>GSHMAAELDSLLGQEKERFQVLPGRDKMLYVAAQNERDTLWARQVLARGDYDKNARVINENEENKRISIWLDTYYPQLAYYRIHFDEPRKPVFWLSRQRNTMSKKELEVLSQKLRALMPYADSVNITLMDDVTAAGQAEAGLKQQALPYSRRNHKGGVTFVIQGALDDVEILRARQFVDSYYRTWGGRYVQFAIELKDDWLKGRSFQYGAEGYIKMSPGHWYFPSPL[2x]

The bacterial injectisome, or type III secretion system (T3SS), is a specialized syringe-shaped protein-export system utilized by many pathogenic Gram-negative bacteria for the injection of virulence proteins (effectors) into host cells. The injectisome can be divided into three major regions: the inner- (IM) and outer-membrane (OM) spanning basal body with associated export apparatus and ATPase components, an extracellular needle, and a terminating pore inserted into the host cell membrane called the translocon. The major structural scaffold of the basal body is comprised largely of three proteins that arrange into a series of highly oligomerized, concentric rings: two intimately associated proteins localized to the IM - PrgK/EscJ/MxiJ and PrgH/EscD/MxiG, and a third protein belonging to the secretin family of OM proteins, InvG/EscC/MxiD (Salmonella enterica serovar Typhimurium SPI-1, Enteropathogenic Escherichia coli (EPEC) LEE and Shigella dysenteriae nomenclature, respectively). In summary, we report the crystal structures for the cytoplasmic and periplasmic domains of PrgH and InvG, two of the main basal body components of the prototypical Salmonella SPI-1 injectisome.

It should be noted that the N-terminal RBMs of PrgH (defined in the new crystal form of PrgH170–392 reported here) and EscJ do not form the conserved oligomerization interface and appear involved in intra-domain interactions or membrane association. No visible density was observed for these residues in the crystal form reported previously, nor in one of the two molecules in the asymmetric unit of the crystal form reported here, suggesting that these residues are flexible. We note that residues 370–392 were not resolved in any of the crystal forms obtained to date, and therefore these residues were not included in any of the modelling attempts. For the periplasmic PrgH170–392 domain, crystallographic symmetry-related molecules in the crystal produce a dimer that exploits the same general interface as the 24-mer biological assembly. Collectively, the crystallographic packing interfaces we observe support and mirror the low energy interfaces generated in our modelled basal body. This would be consistent with a model whereby the soluble domains have low-affinity interaction surfaces for oligomerization, which can be captured by the high concentration in the crystallization experiment. All the reported purified domains of the T3SS basal body are monomeric in solution, showing that the membrane-embedded domains and/or the presence of additional proteins are necessary for their oligomerization.>MGSSHHHHHHSSENLYFQGGGHMTIPFDHWPEWPQHSDRTRRKIEEVFQSNRWAISGYWTGEESMERKFAKAFADFNGVPYCVPTTSGSTALMLALEALGIGEGDEVIVPSLTWIATATAVLNVNALPVFVDVEADTYCIDPQLIKSAITDKTKAIIPVHLFGSMANMDEINEIAQEHNLFVIEDCAQSHGSVWNNQRAGTIGDIGAFSCQQGKVLTAGEGGIIVTKNPRLFELIQQLRADSRVYCDDSSELMHGDMQLVKKGDIQGSNYCLSEFQSAILLDQLQELDDKNAIREKNAMFLNDALSKIDGIKVMKRPPQVSRQTYYGYVFRFDPVKFGGLNADQFCEILREKLNMGTFYLHPPYLPVHKNPLF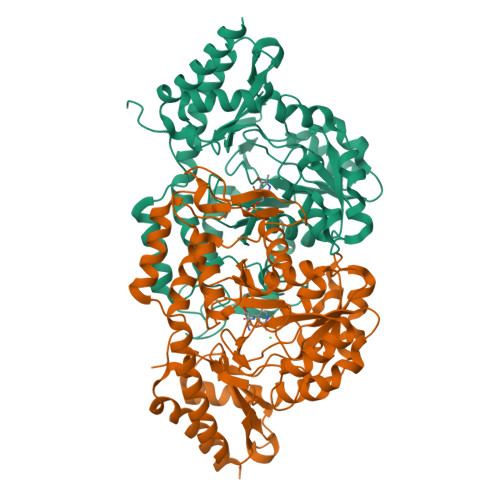CPWTKNRYLKSVRKTEAYWRGLHYPVSERASGQSIVIHHAILLAEPSHLSLLVDAVAELARKFCVTH[2x]4-ethanoyl-3-ethyl-5-methyl-~{N}-(naphthalen-1-ylmethyl)-1~{H}-pyrrole-2-carboxamide 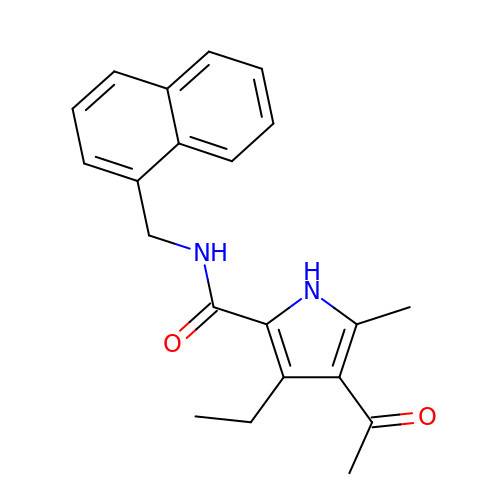| C21 H22 N2 O2 | PDRFAPMZSRHWMA-UHFFFAOYSA-N> MQQGQMAYDRAITVFSPDGRLFQYEYAREAVKKGSTALGMKFANGVLLISDKKVRSRLIEQNSIEKIQLIDDYVAAVT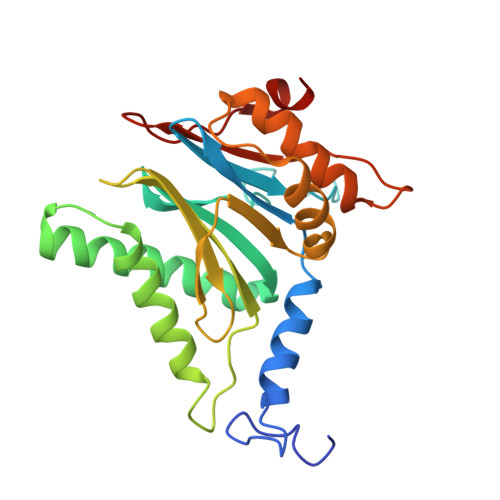SGLVADARVLVDFARISAQQEKVTYGSLVNIENLVKRVADQMQQYTQYGGVRPYGVSLIFAGIDQIGPRLFDCDPAGTINEYKATAIGSGKDAVVSFLEREYKENLPEKEAVTLGIKALKSSLEEGEELKAPEIASITVGNKYRIYDQEEVKKFL>[2x]VSEDLRSRIEVLKRKVIEKVQHIQLLQKNVRAQLVDMKRLEVDIDIKIRSCRGSCSRALAREVDLKDYEDQQKQLEQVIAKDLLPSR;>DNENVVNEYSSELEKHQLYIDETVNSNIPTNLRVLRSILENLRSKIQKLESDVSAQMEYCRTPCTVSCNIPVVSGKECEEIIRKGGETSEMYLIQPDSSVKPYRVYCDMNTENGGWTVIQNRQDGSVDFGRKWDPYKQGFGNVATNTDGKNYCGLPGEYWLGNDKISQLTRMGPTELLIEMEDWKGDKVKAHYGGFTVQNEANKYQISVNKYRGTAGNALMDGASQLMGENRTMTIHNGMFFSTYDRDNDGWLTSDPRKQCSKEDGGGWWYNRCHAANPNGRYYWGGQYTWDMAKHGTDDGVVWMNWKGSWYSMRKMSMKIRPFFPQQ[2x];>KMLEEIMKYEASILTHDSSIRYLQEIYNSNNQKIVNLKEKVAQLEAQ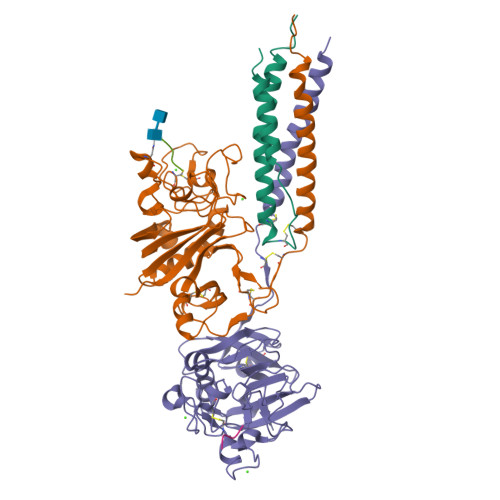CQEPCKDTVQIHDITGKDCQDIANKGAKQSGLYFIKPLKANQQFLVYCEIDGSGNGWTVFQKRLDGSVDFKKNWIQYKEGFGHLSPTGTTEFWLGNEKIHLISTQSAIPYALRVELEDWNGRTSTADYAMFKVGPEADKYRLTYAYFAGGDAGDAFDGFDFGDDPSDKFFTSHNGMQFSTWDNDNDKFEGNCAEQDGSGWWMNKCHAGHLNGVYYQGGTYSKASTPNGYDNGIIWATWKTRWYSMKKTTMKIIPFNRLTIGEGQQHHLGGAKQAGDV[2x];>MHRPY[2x];>GHRP[2x]>[4x]MGSSHHHHHHSSGLVPRGSHMTDLSDVSRTAAAKPPAVPGRGPANKVRFVTAASLFDGHDASINIMRRILQSQGCEVIHLGHNRSVQEVVTAALQEDVQGIAISSYQGGHVEYFKYMIDLLREHGGEHIQVFGGGGGVIVPDEIRELQAYGVARIYSPEDGQRMGLAGMITDMAQRCDIDLTRYAPTTLDTVVAGDRRALAQLITALENGKADPELVSALHAQAKAAAVPVLGITGTGGAGKSSLTDELIRRFRLDQDDALSIAVISIDPSRRKSGGALLGDRIRMNAINHPNIFMRSLATREAGSEISQALPDVIAACKAARFDLVIV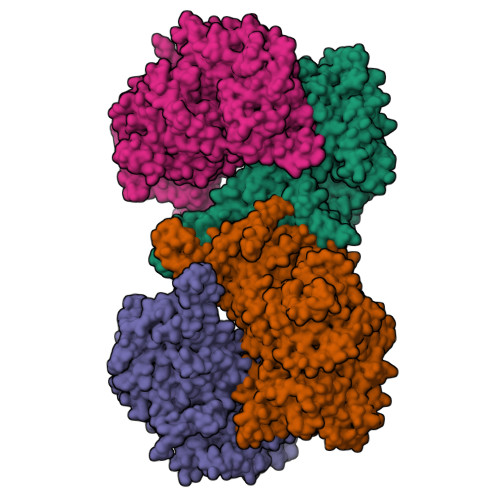ETSGIGQGDAAIVPHVDLSLYVMTPEFGAASQLEKIDMLDFADFVAINKFDRKGAQDAWRDVAKQVQRNREQWHSRAEDMPVYGTQASRFNDDGVTMLYQGLVGALGARGMSLKPGTLPNLEGRISTGQNVIVPPARSRYLAELADTVRAYHRRVVAQSKLARERQQLRAAHDMLQGAGHESAALETLASERDVSLGAVERKLLAMWPQMQQAYSGDEYVVKIRDKEIRTGLISTTLSGTKIRKVVLPRFEDEGEILKWLMRENVPGSFPYTAGVFAFKREGEDPTRMFAGEGDAFRTNRRFKLVSEGMEAKRLSTAFDSVTLYGEDPHERPDIYGKVGNSGVSIATLEDMKVLYDGFDLTNPSTSVSMTINGPAPTILAMFMNTAIDQQIDRFRADNGRDPTADEEAKIRAWVLQNVRGTVQADILKEDQGQNTCIFSTEFSLKVMGDIQEYFVHHQVRNFYSVSISGYHIAEAGANPISQLAFTLANGFTYVEAYLARGMHIDDFAPNLSFFFSNGMDPEYSVLGRVARRIWAVTMRDKYGANDRSQKLKYHIQTSGRSLHAQEIDFNDIRTTLQALIAIYDNCNSLHTNAYDEAITTPTAESVRRALAIQLIINREWGVAKCENPNQGSFLIEELTDLVEEAVLQEFERIAERGGVLGAMETGYQRGKIQEESLYYEQLKHDGTLPIIGVNTFRNPNGDPTPQTLELARSSEDEKQSQLHRLTEFHGAHQADAEAMLARLRQAVIDNRNVFAVLMDAVRVCSLGQITHALFEVGGQYRRNM> SNAPLSFAQQRLWFIAQMSREASGAYHVPGGLRLRGELDEVALRAALDRIMARHEVLRTRFEWHEGEPVQCIDAEARFPLVRQELEGEAAELAHWQQVEARSPFDLGTGPLIRGRLLKLGAQEHVLLLTMHHIVSDGWSMSVLAHELGTLYRAYAQEGTAPE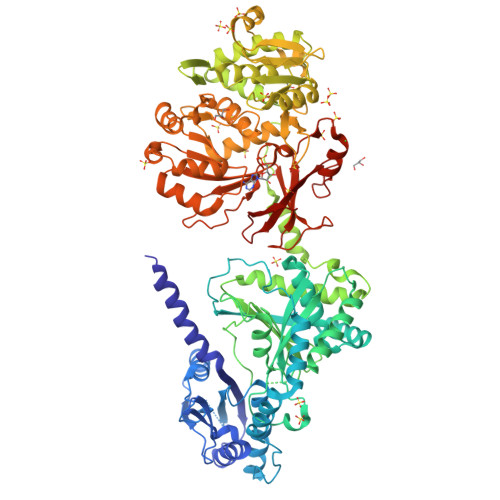VDPLPALPLQYADYALWQRRWLDGERQQRQLAYWQQQLAGAPALVSLPTDRPRPALQDYRGDSIELTFDAGLSQGLRALSQRHGTTLYMTVLAAWAALVARLAGQPEVVIGTPVANRQRAELEGLIGFFVNTLALRVDLGGEPSVAGLLAQVRERVLAAQSHQDLPFEQVVEALKPERSLSHSPVFQLMLSWESSPPHALQMSPLRARPLAPVRERSAQFDLSLHLHEAADGTVAGSLTYASALYERETVQRHAGYLKALLAGMVADDTQPVQRIGILGEAERHRLLVEWNDTAREHPRTVCVHELFEQQVERSPDAVALVYEGQQLSYRELDRQANRLARQLKALGVGPDERVAVCTERCLEMVVALLAVLKAGGAYVPLDPGYPAERLEYMLADSAPKVLLRQSGQTLEPGAGVAVLALDGEASQPWQAQPAQRLSRDDSGVQPHHLAYVIYTSGSTGRPKGVMVEHAGVVNRLLWMQRAYGLQPQEAVLQKTPFGFDVSVWEFFWPLAVGARLVMARPQGQQDPAYLVETIVGQDIGTLHFVPSMLQAFVDSEGVQRCRGVRRIVCSGEALPGALARRLRQQLPQVELHNLYGPTEATVDVTAWACDAAELPDNIPIGRPVDNTTMYVLDAHGQPVPTGVAGEIHIGGVQVARGYLGRPELTRERFVPDPYAGRPGARLYKTGDLGRWLLDGTLEYLGRNDHQVKIRG>[2x]MSRSKRDNNFYSVEIGDSTFTVLKRYQNLKPIGSGAQGIVCAAYDAILERNVAIKKLSRPFQNQTHAKRAYRELVLMKCVNHKNIIGLLNVFTPQKSLEEFQDVYIVMELMDANLCQVIQMELDHERMSYLLYQMLCGIKHLHSAGIIHRDLKPSNIVVKSDCTLKILDFGL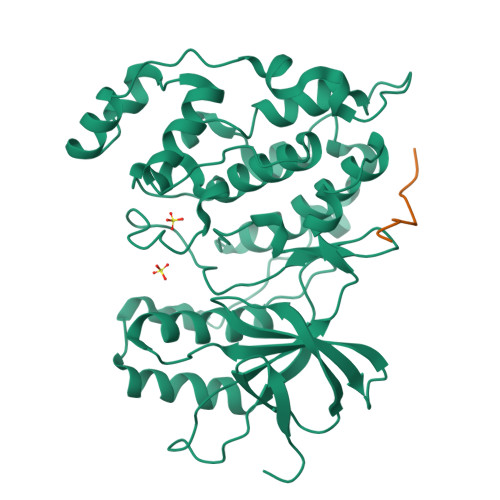ARTAGTSFMMEPEVVTRYYRAPEVILGMGYKENVDIWSVGCIMGEMVCHKILFPGRDYIDQWNKVIEQLGTPCPAFMKKLQPTVRNYVENRPKYAGYSFEKLFPDVLFPADSEHNKLKASQARDLLSKMLVIDASKRISVDEALQHPYINVWYDPSEAEAPPPKIPDKQLDEREHTIEEWKELIYKEVMDLEHHHHHH;>PKRPTTLNLF[2x]>MSAIQASWPSGTECIAKYNFHGTAEQDLPFCKGDVLTIVAVTKDPNWYKAKNKVGREGIIPANYVQKREGVKAGTKLSLMPWFHGKITREQAERLLYPPETGLFLVRESTNYPGDYTLCVSCEGKVEHYRIMYHASKLSIDEEVYFENLMQLVEHYTTDADGLCTRLIKPKVMEGTVAAQDEFYRSGWALNMKELKLLQTIGKGEFGDVMLGDYRGNKVAVKCIKNDATAQAFLAEASVMTQLRHSNLVQLLGVIVEEKGGLYIVTEYMAKGSLVDYLRSRGRSVLGGDCLLKFSLDVCEAMEYLEGNNFVHRDLAARNVLVSEDNVAKV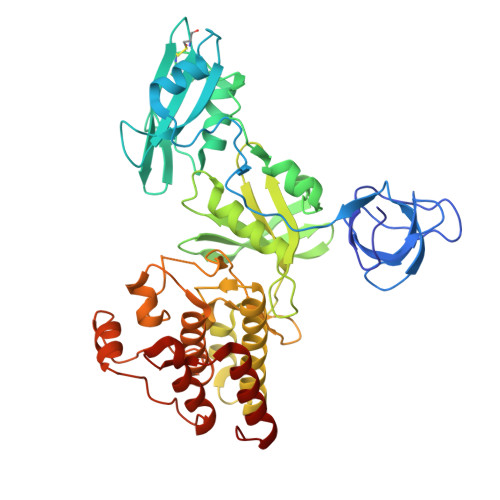SDFGLTKEASSTQDTGKLPVKWTAPEALREKKFSTKSDVWSFGILLWEIYSFGRVPYPRIPLKDVVPRVEKGYKMDAPDGCPPAVYDVMKNCWHLDAATRPTFLQLREQLEHIRTHELHL[6x]> MRDIVFVSPQLYLSSQEGWKSDSAKSGFIPILKNDLQRFQDSLKHIVDARNSLSETLLNSNDDGSIHNSDQNTGLNKDKEASIADNNSANKCATSSSRYQELKQFLPISLDQQIHTVSLQGVSSSFSRGQIESLLDHCLNLALTETQSNSALKVEAWSSFSSFLDTQDIFIRFSKVDEDEAFVNTLNYCKALFAFIRKLHEDFKIELHLDLNTKEYVEDRTGTIPSVKPEKASEFYSVFKNIEDQTDERNSKKEQLDDSSTQYKVDTNTLSDLPSDALDQLCKDIIEFRTKVVSIEKEKKMKSTYEESRRQRHQMQKVFDQIRKNHSGAKGSANTEEEDTNMEDEDEEDDTEDDLALEKRKEERDLEESNRRYEDMLHQLHSNTEPKIKSIRADIMSAENYEEHLE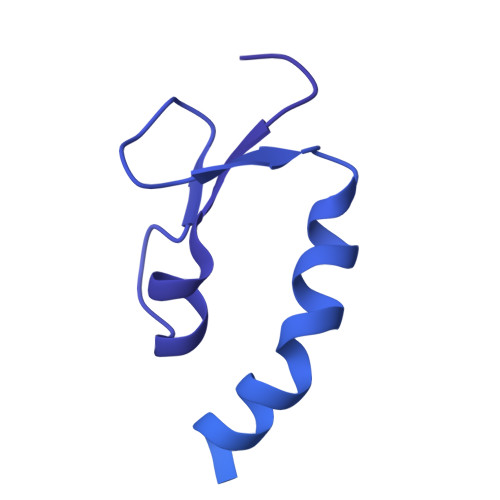KNRSLYLKELLHLANDVHYDHHRSFKEQEERRDEEDRAKNGNAKELAPIQLSDGKAISAGKAAAITLPEGTVKSENYNADKNVSESSEHVKIKFDFKKAIDHSVESSSEDEGYRESELPPTKPSERSAAEDRLPFTADELNIRLTNLKESRYVDELVREFLGVYEDELVEYILENIRVNQSKQALLNELRETFDEDGETIADRLWSRKEFRLGT>[2x]MAHAGRTGYDNREIVMKYIHYKLSQRGYEWDAGDVGAAPPGAAPAPGIFSSQPGHTPHPAASRDPVARTSPLQTPAAPGAAAGPALSPVPPVVHLTLRQAGDDFSRRY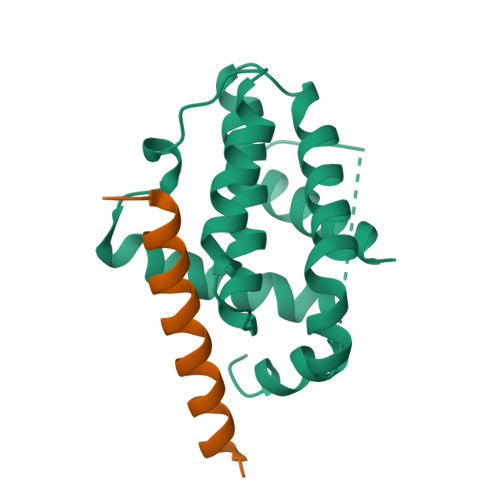RRDFAEMSSQLHLTPFTARGRFATVVEELFRDGVNWGRIVAFFEFGGVMCVESVNREMSPLVDNIALWMTEYLNRHLHTWIQDNGGWDAFVELYGPSMR;>QDASTKKLSECLRRIGDELDSNMELQRMIAD[2x]>[2x]MGSSHHHHHHENLYFQGTTLSSTKVEAPQSTPPSTKIEAPQSKPNATTPPSTKVEAPQQTANATTPPSTKVTTPPSTNTPQPMQSTKSDTPQSPTTKQVPT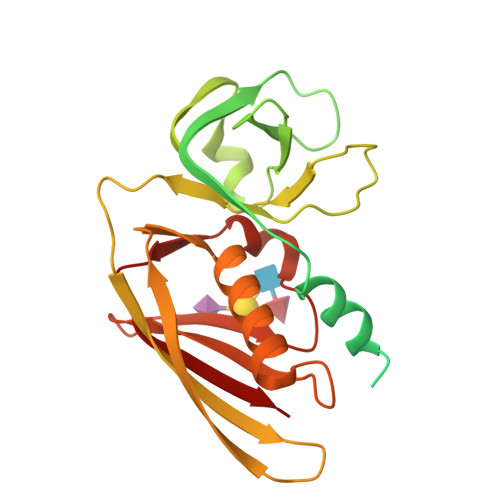EINPKFKDLRAYYTKPSLEFKNEIGIILKKWTTIRFMNVVPDYFIYKIALVGKDDKKYGEGVHRNVDVFVVLEENNYNLEKYSVGGITKSNSKKVDHKAGVRITKEDNKGTISHDVSEFKITKEQISLKELDFKLRKQLIEKNNLYGNVGSGKIVIKMKNGGKYTFELHKKLQENRMADVIDGTNIDNIEVNIK N-(4-{[({(2R)-3-[(3R)-3-amino-4-(2,4,5-trifluorophenyl)butanoyl]-1,3-thiazolidin-2-yl}carbonyl)amino]methyl}phenyl)-D-valine 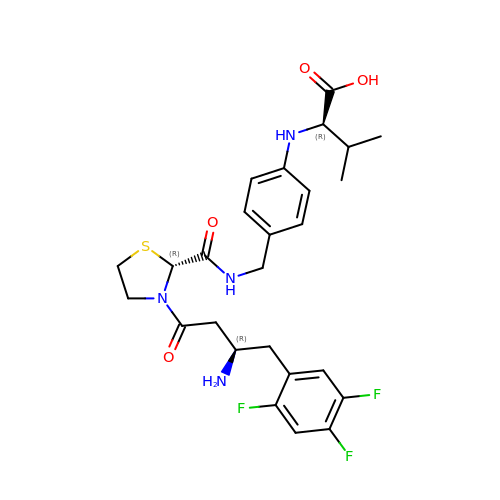| C26 H31 F3 N4 O4 S | ZUNWVBNRQTWJFD-WQWSHVPRSA-N> MADAPVIKNADVAYPSFKGSDDPMKTAANNTTYNPAVSYLQETFDNDVKNLAGIDTDHDFWIDKILTRTGAQPTGKGTNDKGAYSYEGSDGNNYLFTRGRAAYMYTHTPNQLGFVGDTAYWDQTSRSGFTVTVNADGSNQTLNEDASQRKQTPSYFTSLFQTGGKSLKIKEVKYITYNNVMVANLTVESTQDRDVTLTTASPFAAEGADGATELTGRVNVKNNLTTIYPRFSANNQDGSNWIVSGGKLTSTLSLKANEPQTVKIQLGLIANELPDSTKEYEARYTGDLKDAAASYKDSVTTYNKWWVDNAPYVDTPEDNIDKTVVYRWWLSRFNMLDANMPGNTFQYPTSIEGVLGYNNQIVLTSGMFMMDTKWFRNPEYSYGTWLSAGDTAKKSKAGYYYYHDNPGDPANWNHSYTQYITRAGWDSYKVHGGPSTVAEELADQGAEDVQGLLASKSEPDNNDNQNNNDNSLIDWSWWSMTGNDADAVSFSEPGRSGQRMDRADGSANMWANANAAAQAYKAAGDTANAEKMQAIADKIQKEVTTELWDKSDNLLKHKWLNDGAFAKYKEINNYYPYSEGLMPTGNEDYNKALRLFEDSNEFPIFPFFTANQADKAALNFPGSNNFSIINAQPLLQVYSAGIRNYDAAKNGYITNEQFKKLLYWVAFAHYQGGDNNYPDQNEFWNEDNNNVGDVNGDGVINNLDKNLDAAQNGGKITYRSWIHHTQLGTTNWTMVEDVAGMVPREDNKIELNPIEIPGWNYFTVNNLRYHDQDVSIVWDKDGSHYGGPAGYSLYVGGKLAFTSDKLAHLIYDPAAGTVEVKDDSSAQVTVGAEAVKNVKAANQVTFNADQRVTDLFAKSGTNVLEHHHHHH

The GH121 β-L-arabinobiosidase HypBA2 plays a key role in the degradation system by releasing the β-Ara2 that is transferred to the specific sugar importer. HypBA2 is an exo-type glycoside hydrolase that releases a disaccharide (β-Ara2). HypBA2 is a multi-domain protein with 1943 amino acids (aa). In this study, we report the crystal structure of HypBA2 as the first three-dimensional structure of GH121.

The crystal structure of the native (unlabeled) CΔ1049 protein was determined at 1.85 Å resolution. The refined crystal structure of CΔ1049, which contains the core catalytic region of GH121, comprises residues 38–894, and three short regions (residues 438–445, 512–515, and 889–891) were disordered. The overall structure of CΔ1049 consists of a mostly unstructured N-terminal region (residues 38–123, cyan), a N-domain (124–303, marine), a linker region with two α-helices (304–347, orange), a catalytic (α/α)6 barrel domain (348–771, green), a C-domain (772–870, red), and a mostly unstructured C-terminal region with an α-helix (871–894, yellow). The second Ca2+ (Ca2) is located in the A’-region and coordinated by the side chains of Asn497, Asn499, Asn501, Asp505, and Asp532, and the main chain carbonyl of Leu503. The degree of amino acid sequence conservation of GH121 members mapped on the molecular surface of HypBA2 clearly illustrated highly conserved residues in a pocket of the catalytic domain (red). Three conserved acidic residues (Glu383, Asp515, and Glu713) of GH121 (discussed below) and two short disordered regions (438–445 and 512–515) are located in the pocket. Because one of the three conserved acidic residues (Asp515) was disordered in the crystal structure, the neighboring residue (Ala516) is shown with a magenta color in the figures. A triethylene glycol (TEG) molecule, which was derived from the crystallization precipitant, was bound in the pocket (a green stick in Fig 2D). The TEG molecule in the pocket appears to indicate the location of subsite –2. Then, we constructed point mutants of CΔ1049 by site-directed mutagenesis. As shown in Fig 3 (right), mutations of Glu383 and Glu713 (E383A, E383Q, E713A, and E317Q) completely abolished the activity. Based on structural comparisons, we suggest that Glu713 and Asp515 are the likely catalytic nucleophile and acid/base residues of HypBA2, respectively.>GSMGKPFFTRNPSELKGKFIHTKLRKSSRGFGFTVVGGDEPDEFLQIKSLVLDGPAALDGKMETGDVIVSVNDTCVLGHTHAQVVKIFQSIPIGASVDLELCRGYPLGSSAYGSVKAYTNFDAERDALNIETAIKTKGVDEVTIVNILTNRSNEQRQDIAFAYQRRTKKELASALKSALSGHLETVILGLLKTPAQYDASELKASMKGLGTDEDSLIEIICSRTNQELQEINRVYKEMYKTDLEKDIISDTSGDFRKLMVALAKGRRAEDGSVIDYELIDQDARDLYDAGVKRKGTDVPKWISIM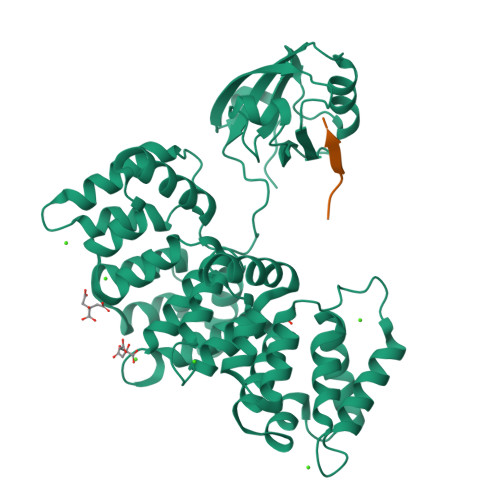TERSVPHLQKVFDRYKSYSPYDMLESIRKEVKGDLENAFLNLVQCIQNKPLYFADRLYDSMKGKGTRDKVLIRIMVSRSEVDMLKIRSEFKRKYGKSLYYYIQQDTKGDYQKALLYLCGGDD[2x];>SSRTRRETQL[2x]> GMPDSPTLLDLFAEDIGHANQLLQLVDEEFQALERRELPVLQQLLGAKQPLMQQLERNGRARAEILREAGVSLDREGLARYARERADGAELLARGDELGELLERCQQANLRNGRIIRANQASTGSLLNILRGQDAPSLYDSRGG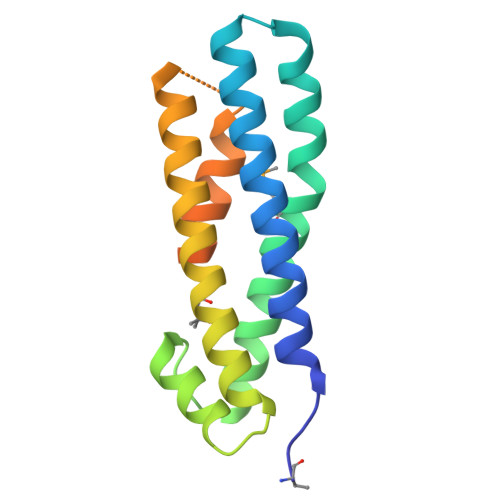TASSSRQRPLSQA> MESYITMNFDKNTAEVGQIIKATVKINKITNFSGYQVNIKYDPTVLQAVNPKTGVAYTNSSLPTSGELLVNEDYGPIVQGVHKISEGILNLSRSYTALDVYRASESPEETGTVAVVGFKALQKKATTVVFEHSVTMPNGIIGTTLFNWYGNRITSGYSVIQPGEINSE;> GTTVSGYINPDFVTTSTTAPIVKAGFTVEIVGTTKSAVTDSNGYFEIKDVAAGTYTVKITKANYLTREIANVSVTADKELSTSASPILMWAGDMAIGGTQDGAINLEDILEICKAFNTSSTDAKYQVGLDLNRDGAISLEDVMIVAKHFGK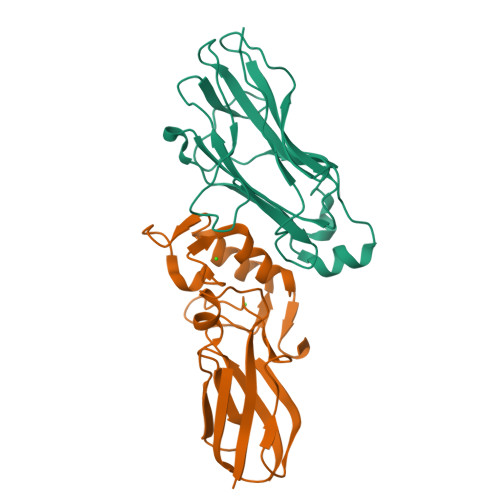VSSDY> L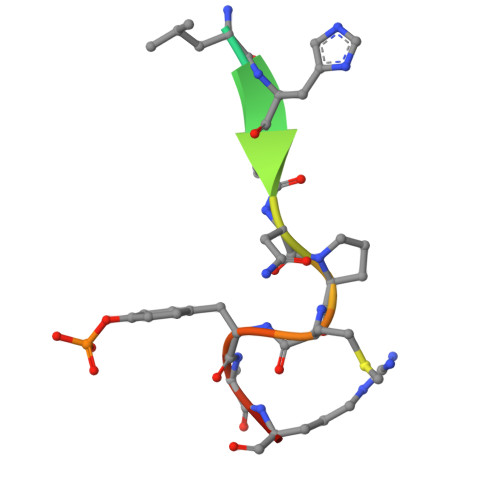DRLHPNPMYQRM By integrating comparative genomics, transcriptomics, functional genetics, and metabolomics analysis, we identified a unique polyyne resistance gene, masL (encoding acetyl-CoA acetyltransferase), in the biosynthesis gene cluster of antifungal polyynes (massilin A 1, massilin B 2, collimonin C 3, and collimonin D 4) of Massilia sp. YMA4. Crystallographic analysis indicated that bacterial polyynes serve as covalent inhibitors of acetyl-CoA acetyltransferase. The monomer of MasL shares the general fold architecture reported in the type II biosynthetic thiolase family. MasL consists of three domains: an N-terminal α/β domain (N-domain, residues 1–121 and 251–271), a loop domain (L-domain, residues 122–250), and a C-terminal α/β domain (C-domain, residues 272–394).

To investigate how bacterial polyynes target acetyl-CoA acetyltransferase, we solved the crystal structures of MasL in its apo and two holo (bound collimonin C 1 and collimonin D 2) forms at 1.78 Å, 1.66 Å, and 1.40 Å resolution, respectively. The asymmetric unit (space group P1 for apo MasL and MasL-collimonin D complex; P21 for MasL-collimonin C complex) of both structures contains a tetramer of the protein, as observed in solution. Although we did not obtain a good X-ray diffraction result surrounding the reactive Cys90 in the MasL-collimonin D complex, the nucleophilic addition mechanism of polyynes to the acetyl-CoA acetyltransferase was confirmed by mass spectrometry analysis. The observation of collimonin C/D (+C16H18O4)–derived adducts of enzyme reactive cysteine residue provided convincing evidence of protein irreversible S-alkylation via nucleophilic addition to the conjugated terminal alkyne. In the further comparative analysis of the polar interactions in the activation pocket of MasL in MasL-collimonin C and MasL-collimonin D complex, the C(7)OH moiety of collimonin C/D 1, 2, His158 of MasL, and a water molecule formed a strong polar interaction network, including a direct hydrogen bond (3.00–3.16 Å) and a water-mediated hydrogen bond between C(7)OH and His158. Furthermore, although there was no significant induced-fit within the pocket, the collimonin C/D 1, 2 caused the Arg135 on the tetramerization loop to swap and form a hydrogen bond interaction and salt bridge, respectively, across the two subunits within the binding site. These polar interacting residues for the collimonin C/D 1, 2 (inhibitor) binding were similar to CoA (product) in other thiolase models. The C6 chiral center of collimonin C/D 1, 2 is critical to forming different polar interactions. In contrast, the C(6)OH of collimonin D 2 did not form a polar interaction network at the contrasting face and showed fixed spatial direction (dihedral angle to C(7)OH from 32.9˚ to 42.6˚).

>[4x]MVKDEIVISSALRTPIGAFSGTLKDTPAAALGAHVVKTLLERTGLAPERVDEVVMGNVLQAGNGMNVARQVAVNGGLPVAVPAHTVNRVCGSGAQAVVTAYAQIRSGLSNLVIAGGVENMDQAPYLMPSLRHGARMGHTQALDALLRDGLNDAFSDQHSGWHTEDLVAKYEVSREAQDRFAATSQQRFAAAQAAGWFEGEIVPVTITTRKGETVFAKDEANRPDTTEAGLAKLRPAFRKDGTITAGNAPGLNAGAAAMIVSSHATATELGLQPQLVIRGIGVAAVEPGLFGFGPVPAIKLALAQAQWQVQDVDRFEVNEAFAAVGLVVRDELGIAPERFNVDGGAIAHGHPIGATGAILLTKVAHALRRTSERRAVVSLCIGGGQGIALALERVKLAAALEHHHHHH>SMTEIRVHQGDLPNLDNYRIDAVAVDTETLGLQPHRDRLCVVQLSSGDGTADVIQIAKGQKSAPNLVRLLSDRDITKIFHFGRFDLAILAHTFGVMPDVVFCTKIASKLTRTYTDRHGLKEICGELLNVNISKQQQSSDWAAETLSRAQIEYAASDVLYLHRLKDIFEERLKREERESVAKACFQFLPMRANLDLLGWSEIDIFAHS[8x]

Orn and NrnC are 3′–5′ exonucleases with a DnaQ fold containing the catalytic DEDD motif, a domain that is common in enzymes that act on nucleic acids. Notably, Orn (and its eukaryotic ortholog REXO2) or NrnC activity is critical for cellular growth, rendering them unique amongst the exoribonucleases known to date. Through quantitative structure-function analyses, we show here that NrnC-type RNases share this narrow substrate length preference with Orn. The structures confirm an octameric assembly as a conserved feature of NrnC-type RNases.

Similar binding poses to pGG at NrnC were observed with pAA and pGC, suggesting that most if not all diribonucleotides can be accommodated by NrnC.GUANOSINE-5'-DIPHOSPHATE-BETA-L-FUCOPYRANOSE 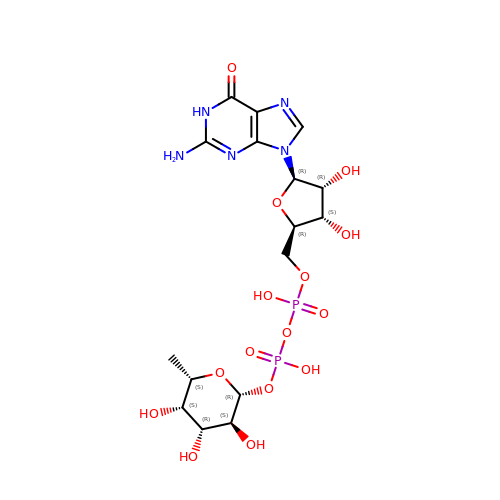| C16 H25 N5 O15 P2 | LQEBEXMHBLQMDB-JGQUBWHWSA-N> GPGGSGGMKPQIRNMVEPMDPRTFVSNFNNRPILSGLDTVWLCCEVKTKDPSGPPLDAKIFQGKVYPKAKYHPEMRFLRWFHKWRQLHHDQEYKVTWYVSWSPCTRCANSVATFLAKDPKVTLTIFVARLYYFWKPDYQQALRILAEAGATMKIMNYNEFQDCWNKFVDGRGKPFKPWNNLPKHYTLLQATLGELLRHLMDPGTFTSNFNNKPWVSGQHETYLCYKVERLHNDTWVPLNQHRGFLRNQAPNIHGFPKGRHAALCFLDLIPFWKLDGQQYRVTCFTSWSPCFSCAQEMAKFISNNEHVSLCIFAARIYDDQGRYQEGLRTLHRDGAKIAMMNYSEFEYCWDTFVDRQGRPFQPWDGLDEHSQALSGRLRAILQNQGN

Human APOBEC3G (hA3G) is a member of apolipoprotein B mRNA editing enzyme catalytic polypeptide like (APOBEC) family, and is one of the most effective antiviral host restriction factors against exogenous retroviral pathogens such as human immunodeficiency virus type 1 (HIV-1) and endogenous retroviral derived remnants on the human genome. hA3G is a DNA/RNA cytidine deaminase converting 3′ target cytidine (C) in 5′-CC-3′ or 5′-CCC-3′ motif to uridine (U) within single-stranded DNA (ssDNA)9–15 or single-stranded RNA (ssRNA). hA3G has two cytidine deaminase domains in tandem, the N-terminal CD1 (or NTD) and C-terminal CD2 (or CTD). The ability to bind nucleic acids and form oligomerization is attributed mainly to CD1/NTD (referred to as CD1 hereafter), while deaminase activity is performed by CD2/CTD (referred to as CD2 hereafter). In this study, we describe four structures of a soluble primate rA3G variant from rhesus macaque, rA3GR8/E259A, in complex with AA and GA dinucleotide-containing RNA molecules in the form of ssRNA and dsRNA with 5′- or 3′-overhangs.

The third complex of rA3G with RNA3-AAxtal was determined as a monomer with one rA3GR8/E259A molecule binding to one ssRNA molecule at 2.10 Å. The electron density of RNA was sufficiently featured for building 6-nt: 5′-U4A5A6U7U8U9-3′ out of the 10-nt 5′-U1U2U3U4A5A6U7U8U9U10-3′. About 47% of the resolved 6-nt ssRNA surface area is buried, with most of the rA3G-ssRNA contacts placed around AA dinucleotides and on the CD1 domain, which is consistent with the findings from the two rA3GR8/E259A-dsRNA complexes described above. 3′A6 in the AA (or A5A6) dinucleotide is bound to an aromatic/hydrophobic “cave”, a pocket outside but right next to the zinc-center of CD1, forming strong hydrophobic interactions with the solvation energy effect of −2.47 kcal/mol. This pocket is largely preformed and comprised of mainly hydrophobic and aromatic residues: 25PILS28 from loop 1, Y59 from loop 3, W94 from loop 5, and 123LYYFW127 from loop 7. Inside the pocket, there are four hydrogen bonds formed (bond lengths 2.8−3.1 Å) between N1, N6, and N7 nitrogen atoms of 3′A6 and the carbonyl and amide groups within CD1-loop 1 (P25, L27, along the Hoogsteen edge of adenine) and loop 7 (L123, Y125, along the Watson–Crick edge of adenine), fitting 3′A6 base snugly into the pocket. 5’A5 in the AA (or A5A6) dinucleotide is bound to a groove conformed by the CD1 and CD2, also forming strong hydrophobic interactions with the solvation energy effect of −3.09 kcal/mol. One hydrogen bond is formed between N6 nitrogen atom of 5’A5 and the main-chain carbonyl group of F268 (bond length 2.8 Å). U4 at the 5’-end of the AA dinucleotide core structure is held between R24 and S28 on the rA3G surface, suggesting a none-base specific binding with the solvation energy effect of 3.05 kcal/mol.>[4x]MNNLTSIDLSPQTLMAMHISISSQALLNQSYSNLLLSQQLLTSQSMDPGLTVKIKAYQNQLRQQAQVFKQNTVA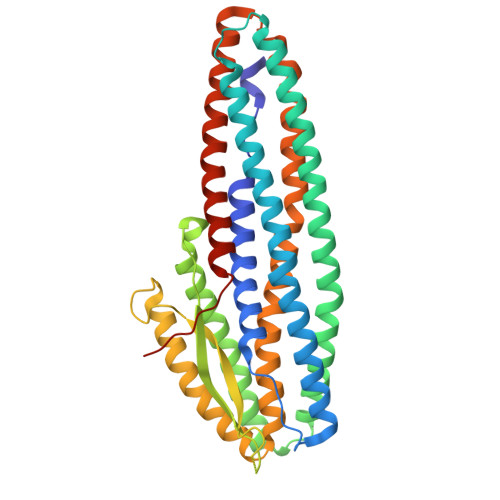ELIGLYTKASNFAALVNAVNALYSTEDPQVSQKGAEMVAALSDVAQHYQAAAQAVHTQLQAKREMLEPLMGNFLNVIDAIEQGLNAEAKQQAQTIAELNEAIAKNIQSIADAGFKAGEGVVQLGQSIVAAVPLGPTDKKPKEAPTAPPKPLSDQASYMISGIQAISAGASGAQQAVNELKANYAKLAVAYRALATANALLSVAKSVQAQAQLFVDTYVLTEQRMALLPTEWGKVAEAYLTAAPIINQAGSAAEIKQAKQIISLNAEKWQLFSKSIDNAKANYAGNNILPEVLEHHHHHH Prokaryotic cells and the chloroplasts of plant cells possess the ribosome-associated chaperone trigger factor, which binds nascent polypeptides at their exit stage from the ribosomal tunnel. The structure of bacterial trigger factor has been well characterized and it has a dragon-shaped conformation, with flexible domains responsible for ribosome binding, peptidyl-prolyl cis–trans isomerization (PPIase) activity and substrate protein binding. In eukaryotic cells, trigger factors are only found in the chloroplasts of plants. Chloroplast trigger factors (hereafter referred to as TIG1s) display a remarkable sequence variance compared with prokaryotic TFs, while the typical organization of the three domains remains conserved.

Here, the crystal structure of the plastidic trigger factor from the green alga Chlamydomonas reinhardtii is presented at 2.6 Å resolution. Due to the high intramolecular flexibility of the protein, diffraction to this resolution was only achieved using a protein that lacked the N-terminal ribosome-binding domain. The resulting atomic structure of CrTIG1 lacks the first 137 amino acids of the mature protein (without the chloroplast signal peptide) and will be referred to here as CrTIG1ΔRBD. Visible electron density starts with amino acid Val138 at the beginning of the linker region between the N-terminal RBD and the middle PPIase domain, with β5 being the first secondary-structure element. The protein resembles the dragon-like structure described for bacterial trigger factors, but without the tail (the RBD). The PPIase domain, which forms the head of the dragon-like structure, is prominently tilted downwards in CrTIG1ΔRBD towards the arms. The C-terminal domain of CrTIG1 stands out by its unique features and differently arranged arms, which are not found in bacterial trigger factors. The arms are oriented towards each other and do not show the prominent ‘open arms’ conformation of the bacterial trigger factors, which build a cavity for substrate protein binding. Comparison of both chains in the asymmetric unit of the crystal structure shows differences in the position of arm 1 but smaller differences in arm 2. Indeed, we measured a PPIase activity of CrTIG1 of 0.0057 µM −1 s−1, which is 100-fold lower than that of EcTF with the substrate, but still measurable and within the range of other plant FKBP proteins.

>[2x]AAAGKEKDVKVEVSVAVEELGTCSRSAIITVPASTVKDIFKRGVKRIERDVVGQLKGWQAGKPLPLSMVIQQVGGQNKFKTFCLEELLLEALPKGIESARNGRAVDPASVTVPPEDFPSMLERYDPAKEFFFRAMFDVAPPVVWRTPLEELEVTIRDTGDFSTDAAAADDLIRQYRKQHGFSRVVAGRGLQLGDTLVIDLEITSKATGQALPGLTHKRFSFDTEADVLGITSGMLGMKAGESRTFNMSMPEDYDVEFWQSMPVKVAAKVHEIFEWTLPEFNDEYVAKQHEGKWGSAKEMREALIASTAMQRVTELDKALEDAVVKAVADALDMPEVPPRMVEQLGERQFQAQLLQMIEDRIGSREDVEKLATEEMAAEFIRERKKDLEDQVKFNLAVDDIWVRKGLVLEDEAVEAEFSLRARQMEAVGQPFDREDMLDDVRETVKSVTVIEWLKDNVKRHVLPYTAADDKAAKAKGEPVAV>GMQTQDYQALDRAHHLHPFTDFKALGEEGSRVVTHAEGVYIHDSEGNRILDGMAGLWCVNLGYGRRELVEAATAQLEQLPYYNTFFKTTHPPAVRLAEKLCDLAPAHINRVFFTGSGSEANDTVLRMVRRYWALKGQPDKQWIIGRENAYHGSTLAGMSLGGMAPMHAQGGPCVPGIAHIRQPYWFGEGRDMSPEAFGQTCAEALEEKILELGEEKVAAFIAEPVQGAGGAIMPPESYWPAVKKVLAKYDILLVADEVI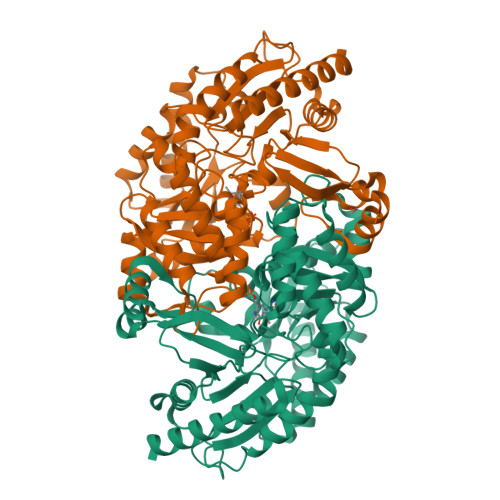CGFGRLGEWFGSQHYGLEPDLMPIAKGLSSGYLPIGGVLVGDRVAETLIEEGGEFFHGFTYSGHPTCAAVALKNLELLEAEGVVDRVRDDLGPYLAERWASLVDHPIVGEARSLGLMGALELVADKTTGQRFDKSLGAGNLCRDLCFANGLVMRSVGDTMIISPPLVIRREEIDELVELARRALDETARQLTQVPHTQEEPTA[2x]> MFLYNLTLQRATGISFAIHGNFSGTKQQEIVVSRGKILELLRPDPNTGKVHTLLTVEVFGVIRSLMAFRLTGGTKDYIVVGSDSGRIVILEYQPSKNMFEKIHQETFGKSGCRRIVPGQFLAVDPKGRAVMISAIEKQKLVYILNRDAAARLTISSPLEAHKANTLVYHVVGVDVGFENPMFACLEMDYEEADNDPTGEAAANTQQTLTFYELDLGLNHVVRKYSEPLEEHGNFLITVPGGSDGPSGVLICSENYITYKNFGDQPDIRCPIPRRRNDLDDPERGMIFVCSATHKTKSMFFFLAQTEQGDIFKITLETDEDMVTEIRLKYFDTVPVAAAMCVLKTGFLFVASEFGNHYLYQIAHLGDDDEEPEFSSAMPLEEGDTFFFQPRPLKNLVLVDELDSLSPILFCQIADLANEDTPQLYVACGRGPRSSLRVLRHGLEVSEMAVSELPGNPNAVWTVRRHIEDEFDAYIIVSFVNATLVLSIGETVEEVTDSGFLGTTPTLSCSLLGDDALVQVYPDGIRHIRADKRVNEWKTPGKKTIVKCAVNQRQVVIALTGGELVYFEMDPSGQLNEYTERKEMSADVVCMSLANVPPGEQRSRFLAVGLVDNTVRIISLDPSDCLQPLSMQALPAQPESLCIVEMGGTEKQDELGERGSIGFLYLNIGLQNGVLLRTVLDPVTGDLSDTRTRYLGSRPVKLFRVRMQGQEAVLAMSSRSWLSYSYQSRFHLTPLSYETLEFASGFASEQCPEGIVAISTNTLRILALEKLGAVFNQVAFPLQYTPRKFVIHPESNNLIIIETDHNAYTEATKAQRKQQMAEEMVEAAGEDERELAAEMAAAFLNENLPESIFGAPKAGNGQWASVIRVMNPIQGNTLDLVQLEQNEAAFSVAVCRFSNTGEDWYVLVGVAKDLILNPRSVAGGFVYTYKLVNNGEKLEFLHKTPVEEVPAAIAPFQGRVLIGVGKLLRVYDLGKKKLLRKCENKHIANYISGIQTIGHRVIVSDVQESFIWVRYKRNENQLIIFADDTYPRWVTTASLLDYDTVAGADKFGNICVVRLPPNTNDEVDEDPTGNKALWDRGLLNGASQKAEVIMNYHVGETVLSLQKTTLIPGGSESLVYTTLSGGIGILVPFTSHEDHDFFQHVEMHLRSEHPPLCGRDHLSFRSYYFPVKNVIDGDLCEQFNSMEPNKQKNVSEELDRTPPEVSKKLEDIRTRYAF;> MTDRYTIHSQLEHLQSKYIGTGHADTTKWEWLVNQHRDSYCSYMGHFDLLNYFAIAENESKARVRFNLMEKMLQPCGPPADKPEEN;> MAKIAKTHEDIEAQIREIQGKKAALDEAQGVGLDSTGYYDQEIYGGSDSRFAGYVTSIAATELEDDDDDYSSSTSLLGQKKPGYHAPVALLNDIPQSTEQYDPFAEHRPPKIADREDEYKKHRRTMIISPERLDPFADGGKTPDPKMNARTYMDVMREQHLTKEEREIRQQLAEKAKAGELKVVNGAAASQPPSKRKRRWDQTADQTPGATPKKLSSWDQAETPGHTPSLRWDETPGRAKGSETPGATPGSKIWDPTPSHTPAGAATPGRGDTPGHATPGHGGATSSARKNRWDETPKTERDTPGHGSGWAETPRTDRGGDSIGETPTPGASKRKSRWDETPASQMGGSTPVLTPGKTPIGTPAMNMATPTPGHIMSMTPEQLQAWRWEREIDERNRPLSDEELDAMFPEGYKVLPPPAGYVPIRTPARKLTATPTPLGGMTGFHMQTEDRTMKSVNDQPSGNLPFLKPDDIQYFDKLLVDVDESTLSPEEQKERKIMKLLLKIKNGTPPMRKAALRQITDKAREFGAGPLFNQILPLLMSPTLEDQERHLLVKVIDRILYKLDDLVRPYVHKILVVIEPLLIDEDYYARVEGREIISNLAKAAGLATMISTMRPDIDNMDEYVRNTTARAFAVVASALGIPSLLPFLKAVCKSKKSWQARHTGIKIVQQIAILMGCAILPHLRSLVEIIEHGLVDEQQKVRTISALAIAALAEAATPYGIESFDSVLKPLWKGIRQHRGKGLAAFLKAIGYLIPLMDAEYANYYTREVMLILIREFQSPDEEMKKIVLKVVKQCCGTDGVEANYIKTEILPPFFKHFWQHRMALDRRNYRQLVDTTVELANKVGAAEIISRIVDDLKDEAEQYRKMVMETIEKIMGNLGAADIDHKLEEQLIDGILYAFQEQTTEDSVMLNGFGTVVNALGKRVKPYLPQICGTVLWRLNNKSAKVRQQAADLISRTAVVMKTCQEEKLMGHLGVVLYEYLGEEYPEVLGSILGALKAIVNVIGMHKMTPPIKDLLPRLTPILKNRHEKVQENCIDLVGRIADRGAEYVSAREWMRICFELLELLKAHKKAIRRATVNTFGYIAKAIGPHDVLATLLNNLKVQERQNRVCTTVAIAIVAETCSPFTVLPALMNEYRVPELNVQNGVLKSLSFLFEYIGEMGKDYIYAVTPLLEDALMDRDLVHRQTASAVVQHMSLGVYGFGCEDSLNHLLNYVWPNVFETSPHVIQAVMGALEGLRVAIGPCRMLQYCLQGLFHPARKVRDVYWKIYNSIYIGSQDALIAHYPRIYNDDKNTYIRYELDYIL;> MAKHHPDLIFCRKQAGVAIGRLCEKCDGKCVICDSYVRPCTLVRICDECNYGSYQGRCVICGGPGVSDAYYCKECTIQEKDRDGCPKIVNLGSSKTDLFYERKKYGFKKR;> AAAAARAARAAAWRAEQAAAA;> MATEHPEPPKAELQLPPPPPPGHYGAWAAQELQAKLAEIGAPIQGNREELVERLQSYTRQTGIVLNRPVLRGEDGDKAAPPPMSAQLPGIPMPPPPLGLPPLQPPPPPPPPPPGLGLGFPMAHPPNLGPPPPLRVGEPVALSEEERLKLAQQQAALLMQQEERAKQQGDHSLKEHELLEQQKRAAVLLEQERQQEIAKMGTPVPRPPQDMGQIGVRTPLGPRVAAPVGPVGPTPTVLPMGAPVPRPRGPPPPPGDENREMDDPSVGPKIPQALEKILQLKESRQEEMNSQQEEEEMETDARSSLGQSASETEEDTVSVSKKEKNRKRRNRKKKKKPQRVRGVSSESSGDREKDSTRSRGSDSPAADVEIEYVTEEPEIYEPNFIFFKRIFEAFKLTDDVKKEKEKEPEKLDKLENSAAPKKKGFEEEHKDSDDDSSDDEQEKKPEAPKLSKKKLRRMNRFTVAELKQLVARPDVVEMHDVTAQDPKLLVHLKATRNSVPVPRHWCFKRKYLQGKRGIEKPPFELPDFIKRTGIQEMREALQEKEEQKTMKSKMREKVRPKMGKIDIDYQKLHDAFFKWQTKPKLTIHGDLYYEGKEFETRLKEKKPGDLSDELRISLGMPVGPNAHKVPPPWLIAMQRYGPPPSYPNLKIPGLNSPIPESCSFGYHAGGWGKPPVDETGKPLYGDVFGTNAAEFQTKTEEEEIDRTPWGELEPSDEESSEEEEEEESDEDKPDETGFITPADSGLITPGGFSSVPAGMETPELIELRKKKIEEAMDGSETPQLFTVLPEKRTATVGGAMMGSTHIYDMSTVMSRKGPAPELQGVEVALAPEELELDPMAMTQKYEEHVREQQAQVEKEDFSDMVAEHAAKQKQKKRKAQPQDSRGGSKKYKEFKF;> MAAGPISERNQDATVYVGGLDEKVSEPLLWELFLQAGPVVNTHMPKDRVTGQHQGYGFVEFLSEEDADYAIKIMNMIKLYGKPIRVNKASAHNKNLDVGANIFIGNLDPEIDEKLLYDTFSAFGVILQTPKIMRDPDTGNSKGYAFINFASFDASDAAIEAMNGQYLCNRPITVSYAFKKDSKGERHGSAAERLLAAQNPLSQADRPHQLFADAPPPPSAPNPVVSSLGSGLPPPGMPPPGSFPPPVPPPGALPPGIPPAMPPPPMPPGAAGHGPPSAGTPGAGHPGHGHSHPHPFPPGGMPHPGMSQMQLAHHGPHGLGHPHAGPPGSGGQPPPRPPPGMPHPGPPPMGMPPRGPPFGSPMGHPGPMPPHGMRGPPPLMPPHGYTGPPRPPPYGYQRGPLPPPRPTPRPPVPPRGPLRGPLPQ;> MDFQHRPGGKTGSGGVASSSESNRDRRERLRQLALETIDINKDPYFMKNHLGSYECKLCLTLHNNEGSYLAHTQGKKHQTNLARRAAKEAKEAPAQPAPEKVKVEVKKFVKIGRPGYKVTKQRDSEMGQQSLLFQIDYPEIAEGIMPRHRFMSAYEQRIEPPDRRWQYLLMAAEPYETIAFKVPSREIDKAEGKFWTHWNRETKQFFLQFHFKMEKPPAPPSLPAGPPGVKRPPPPLMNGLPPRPPLPESLPPPPPGGLPLPPMPPTGPAPSGPPGPPQLPPPAPGVHPPAPVVHPPASGVHPPAPGVHPPAPGVHPPAPGVHPPTSGVHPPAPGVHPPAPGVHPPAPGVHPPAPGVHPPAPGVHPPPSAGVHPQAPGVHPAAPAVHPQAPGVHPPAPGMHPQAPGVHPQPPGVHPSAPGVHPQPPGVHPSNPGVHPPTPMPPMLRPPLPSEGPGNIPPPPPTN;> METILEQQRRYHEEKERLMDVMAKEMLTKKSTLRDQINSDHRTRAMQDRYMEVSGNLRDLYDDKDGLRKEELNAISGPNEFAEFYNRLKQIKEFHRKHPNEICVPMSVEFEELLKARENPSEEAQNLVEFTDEEGYGRYLDLHDCYLKYINLKASEKLDYITYLSIFDQLFDIPKERKNAEYKRYLEMLLEYLQDYTDRVKPLQDQNELFGKIQAEFEKKWENGTFPGWPKETSSALTHAGAHLDLSAFSSWEELASLGLDRLKSALLALGLKCGGTLEERAQRLFSTKGKSLESLDTSLFAKNPKSKGTKRDTERNKDIAFLEAQIYEYVEILGEQRHLTHENVQRKQARTGEEREEEEEEQISESESEDEENEIIYNPKNLPLGWDGKPIPYWLYKLHGLNINYNCEICGNYTYRGPKAFQRHFAEWRHAHGMRCLGIPNTAHFANVTQIEDAVSLWAKLKLQKASERWQPDTEEEYEDSSGNVVNKKTYEDLKRQGLL

Splicing modulators alter the splicing patterns in cells by binding to the U2 snRNP (small nuclear ribonucleoprotein)—a complex chaperoning the selection of branch and 3′ splice sites. The U2 snRNP has a bipartite organization, exhibiting a smaller U2 3′ module and a larger U2 5′ module. The latter contains the heptameric SF3B complex, whose core subunit SF3B1 is recurrently mutated in cancers. In this work, by employing FR901464 analogs as molecular tools to dissect the splicing pathway, we elucidate how spliceostatins/sudemycins interfere with prespliceosome assembly and splicing commitment by covalent coupling to a reactive zinc finger of PHF5A.

To elucidate the impact of antitumor splicing modulators on the splicing pathway and reveal how the U2 snRNP accurately selects and binds the introns, we set out to obtain the cryo-EM structure of a prespliceosome arrested by SSA. We designed a model RNA substrate consisting of 54 intron nucleotides, the second MINX exon, the downstream 5′SS, and three MS2 aptamers for affinity purification. Single-particle cryo-EM analysis of A3′-SSA enabled the reconstruction of a ~12 Å density map that corresponds to the U2 snRNP module of the complex. Focused classification and refinement enabled us to resolve the U2 5′ module to a resolution of ~3.1 Å. In this map, we modeled the SF3B complex, the two matrin-type zinc-finger domains of SF3A2 and SF3A3, part of the intron substrate paired to the U2 snRNA, and the SSA ligand used to arrest the splicing reaction. SSA has an elongated, L-shaped density and is positioned in the hinged pocket of SF3B, between its SF3B1 and PHF5A subunits. Equally unexpected, U2 pairs with the intron, despite SSA having bound to the open state of SF3B. The structure of the A3′-SSA captures an E-to-A intermediate, indicating how the U2/intron duplex forms in at least two steps. The structure of A3′-SSA shows that SSA’s binding to the hinged pocket allows the initial U2-intron pairing in the form of the precursor duplex while preventing its further extension. The A3′-SSA structure reveals that FR901464 analogs, such as SSA or SD6, act at the latest stages of intron selection by the U2 snRNP by “locking” the SF3B1 subunit in an open state and preventing the formation of the extended U2/intron duplex.6-[(cyclopropanecarbonyl)amino]-N-methyl-4-{[2-(methylsulfonyl)phenyl]amino}pyridine-3-carboxamide | C18 H20 N4 O4 S 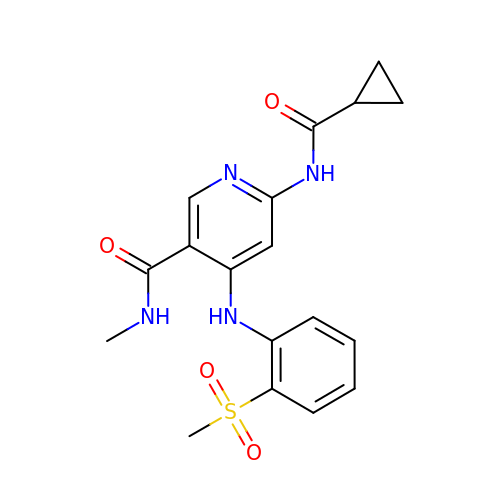| YGFJMLGZTAWLOO-UHFFFAOYSA-N> GSHMRRLQQTQAQVDEVVDIMRVNVDKVLERDQKLSELDDRADALQAGASQFETSAAKLKRKYWWKNLKM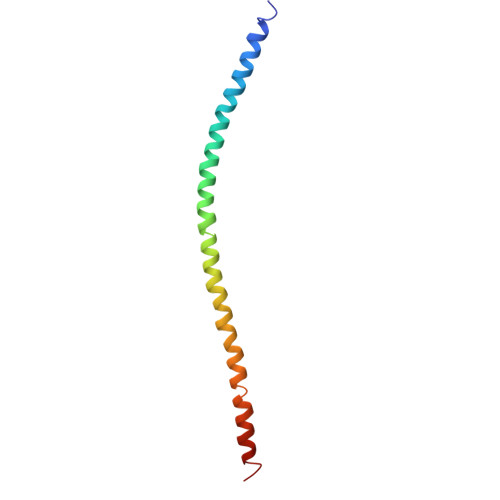MIILGVICAIILIIIIVYFST Secondary structures formed by expanded CUG RNA are involved in the pathobiology of myotonic dystrophy type 1. Of these repeats, CUG repeat RNA expansion in the 3′-untranslated region of dystrophia myotonica protein kinase mRNA has been shown to play an important role in the pathogenesis of DM1 (24, 25). The expanded CUG RNA forms a hairpin structure and binds the muscleblind like splicing regulator 1 (MBNL1) protein, resulting in splicing defects in the insulin receptor and muscle main chloride ion-related pre-mRNAs. The two RNA duplexes exhibit end-to-end stacking to generate infinite pseudocontinuous CUG helices, which resemble the stem structure of stem-loops known to form in long CUG repeats.

To reveal the structural impact of U–U mismatches in CUG repeats, we determined the crystal structure of a 13-mer RNA nucleotide consisting of three continuous CUG repeats in a trigonal space group P3221. The biological assembly formed an intermolecular duplex in the crystal, while the asymmetric unit contains only a single RNA strand, indicating a 2-fold crystallographic symmetry. This RNA is denoted as M3 duplex in the following discussion. The first and third mismatches exhibit a mirror isoform, asymmetric, single hydrogen bonded geometry in which one of the uridines is tilted into the minor groove (MM1 and MM2 states). On the other hand, the central U7–U20 mismatch in the M3 crystal structure shows a unique symmetrical conformation with no inclination of the two uridines (MMT type). The values for the λ-angle are about 72° for both uridine bases within the mismatch. Moreover, the base pair opening is about 35°, resulting in a large distance between the carbonyl oxygen and the N3 amino group of the two uridine residues, so there is no direct hydrogen bonding. In the M3 structure, the U7–U20 mismatch pair showed a unique planar water-bridged interaction. Another water bridges the interactions between two N3 amino atoms of two uridine residues with a short intermolecular distance of 2.9 Å. In the M3 structures, the central symmetric U–U mismatch shows a high stretch and high opening angle, which pushes two uridines away from each other. This particular situation resulted in a single-sided cross-strand stacking of one of the uridines (U7) with C6–G21, while another uridine (U20) is stacked with base pair C19–G8.

> UUCUGCUGCUGAA>MVNVAVIGAAGGIGQSLSLLLLRELPFGSTLSLYDVVGAPGVAADLSH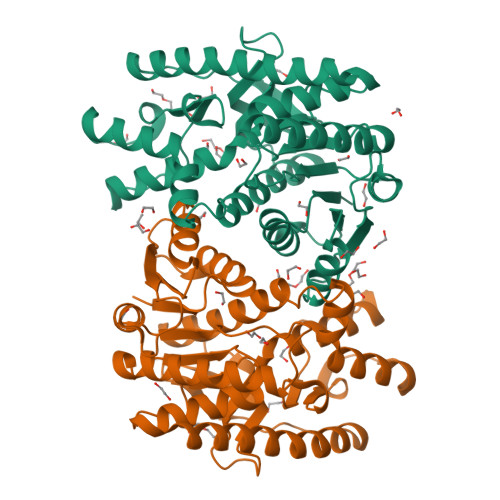IDRAGITVKHAAGKLPPVPRDPALTELAEGVDVFVIVAGVPRKPGMTRDDLFNVNAGIVMDLVLTCASVSPNACFCIVTNPVNSTTPIAAQTLRKIGVYNKNKLLGVSLLDGLRATRFINNARHPLVVPYVPVVGGHSDVTIVPLYSQIPGPLPDESTLKEIRKRVQVAGTEVVKAKAGRGSATLSMAEAGARFTMHVVKALMGLDTPMVYAYVDTDGEHECPFLAMPVVLGKNGIERRLPIGPITTVEKEMLEEAVGVVKKNIAKGETFARSKL[8x]>TAPSQVLKIRRPDDWHLHLRDGDMLKTVVPYTSEIYGRAIVMPNLAPPVTTVEAAVAYRQRILDAVPAGHDFTPLMTCYLTDSLDPNELERGFNEGVFTAAKLYPANATVNSSHGVTSVDAIMPVLERMEKIGMPLLVHGEVTHADIDIFDREARFIESVMEPLRQRLTALKVVFEHITTKDAADYVRDGNERLAATITPQHLMFNRNHMLVGGVRPHLYCLPILKRNIHQQALRELVASGFNRVFLGTDSAPHARHRKESSCGCAGCFNAPTALGSYATVFEEMNALQHFE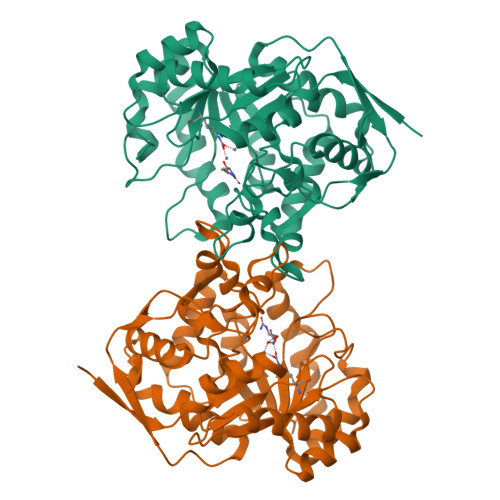AFCSVNGPQFYGLPVNDTFIELVREEQQVAESIALTDDTLVPFLAGETVRWSVKQ[2x]> FPTIPLSRLFDNAMLRAHRLHQLAFDTYQEFEEAYIPKEQKYSFLQNPQTSLCFSESIPTPSNREETQQKSNLELLRISLLLIQSWLEPVQFLRSVFANSLVYGASDSNVYDLLKDLEERIQTLMGRLEDGSPRTGQIFKQTYSKFDTNSHNDDALLKNYGLLYCFRKDMDKVETFLRIVQCRSVEGSCGF;> QLPPGK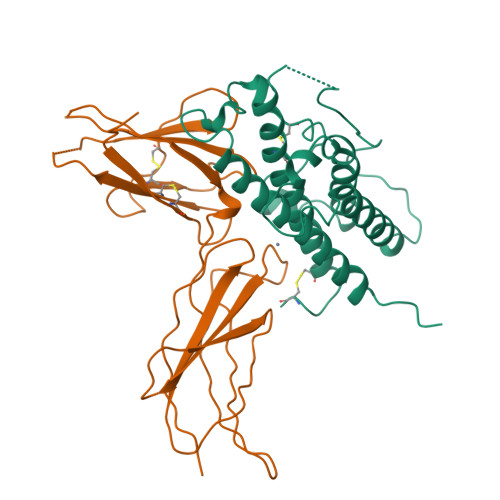PEIFKCRSPNKETFTCWWRPGTDGGLPTNYSLTYHREGETLMHECPDYITGGPNSCHFGKQYTSMWRTYIMMVNATNQMGSSFSDELYVDVTYIVQPDPPLELAVEVKQPEDRKPYLWIKWSPPTLIDLKTGWFTLLYEIRLKPEKAAEWEIHFAGQQTEFKILSLHPGQKYLVQVRCKPDHGYWSAWSPATFIQIPSDFTMNDT>HDTTVFQGVAGQSLQVSCPYDSMKHWGRRKAWCRQLGEK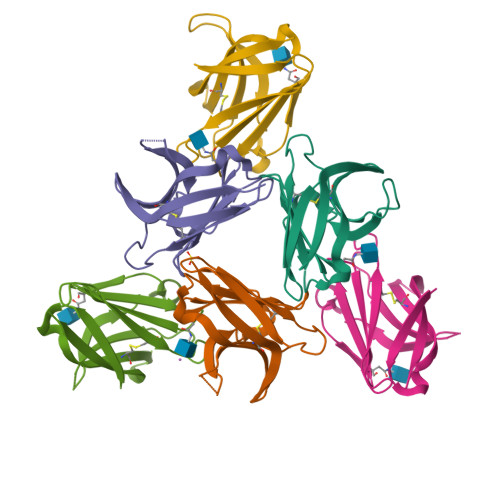GPCQRVVSTHNLWLLSFLRRWNGSTAITDDTLGGTLTITLRNLQPHDAGLYQCQSLHGSEADTLRKVLVEVLADPLDHRDAGDLWFPGESESFEDAHVEHSISRSLLEGEIPFPPTSENLYFQGHHHHHH[6x]> NESSPLHMGAGSANWTAVAR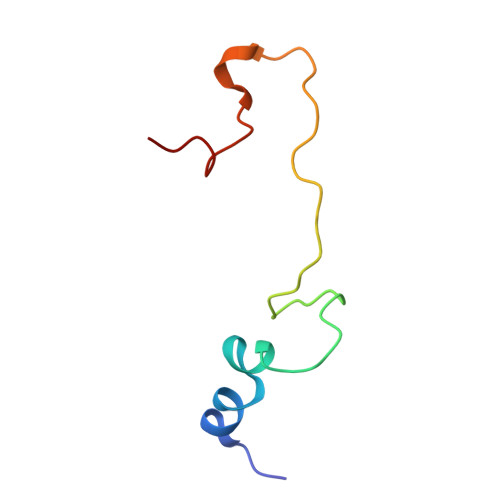LEDFTLRGLSHPPWIHVSSRPFYGAGGGAVLAACMSSAVW>MPVPNGATFPPCARKMERADGPATVLAIGTANPPNVFDQSTYPDFYFNITNSNHMTDLKTKFQRMCDKSGITKRYMYLNEEILKANPNMCAYWEKSLDVRQDMVVVEVPKLGKEAATKAIKEWGQPKSKITHVVFCTTSGVDMPGADWALTKLLGLRPSVKRLMMYQQGCFAGGTVMRVAKDLAENNKGARVLVVCSELTAVTFRGPSETHLDSLVGQALFGDGASAIIVGADPIPEVERPWFEIHYVASNILPDSDGAIDGHLREVGLTFHLMKDVPGIISKNIGTVLKDAFEKVFGNEEGEVPSYNDVFWIAHPGGPAILDQVEQKLQLKTEKMAASRQVLSDYGNMSSACVLFIMDHLRKKSVEQKLATSGEGYEWGLLLGFGPGLTCETVVLRSVPLATE[4x]

Chalcone synthase, a well-studied ubiquitous plant-specific type III polyketide synthases (PKSs), is the first key enzyme in the flavonoid biosynthetic pathway. The biosynthesis of flavonoids starts with the condensation of one molecule of p-coumaryl CoA with three molecules of malonyl-CoA through the catalysis of chalcone synthase (CHS) to generate naringenin chalcone. Functional characterization of two chalcone synthases (CpCHS1 and CpCHS2) indicated that CpCHS1 can catalyze the formation of pinocembrin, naringenin, and eriodictyol, respectively; however, CpCHS2 was inactive. The crystallization investigation of CpCHS1 indicated that it has a highly similar conformation and shares a similar general catalytic mechanism to other plants CHSs.

The crystal structure of CpCHS1 was elucidated in the apo and presence of its final product naringenin, and detailed structural comparisons of CpCHS1 with EaCHS from Equisetum arvense and PpCHS from Physcomitrella patens revealed common differences between CHSs in the local conformation around the active site pocket. And by site-directed mutagenesis, we found seven residues, especially Leu199 and Thr203 that are critical to the catalytic activity for CpCHS1.>[2x]SSTHPVFHMGEFSVCDSVSVWVGDKTTATDIKGKEV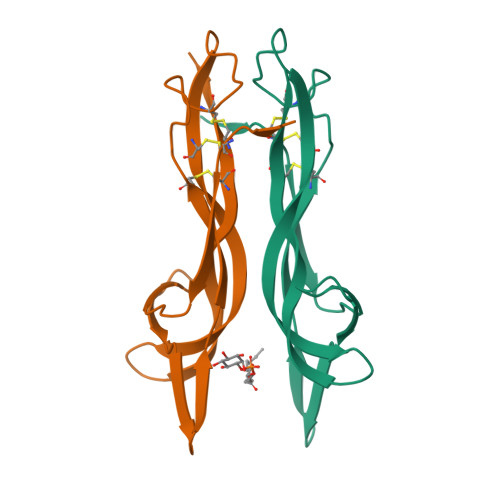TVLAEVNINNSVFRQYFFETKCRASNPVESGCRGIDSKHWNSYCTTTHTFVKALTTDEKQAAWRFIRIDTACVCVLSRKATRRG> AEGDDPAKAAFDSLQASATEYIG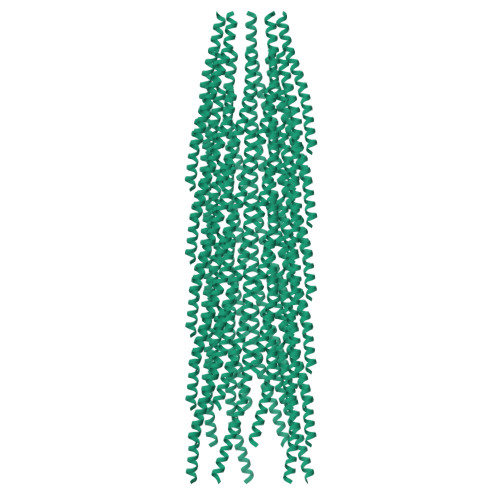YAWAMVVVIVGATIGIKLFKKFTSKAS3-ethoxybenzene-1-carboximidamide 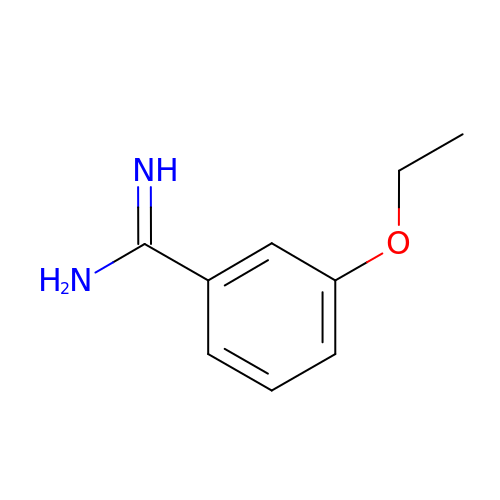| C9 H12 N2 O | OZPMVTBYBADRPR-UHFFFAOYSA-N>[3x]MEITTLQIVLVFIVACIAGMGSILDEFQFHRPLIACTLVGIVLGDMKTGIIIGGTLEMIALGWMNIGAAVAPDAALASIISTILVIAGHQSIGAGIALAIPLAAAGQVLTIIVRTITVAFQHAADKAADNGNLTAISWIHVSSLFLQAMRVAIPAVIVALSVGTSEVQNMLNAIPEVVTNGLNIAGGMIVVVGYAMVINMMRAGYLMPFFYLGFVTAAFTNFNLVALGVIGTVMAVLYIQLSPKYNRVAGAPAQAAGNNDLDNELDHHHHHHHH;>MVDTTQTTTEKKLTQSDIRGVFLRSNLFQGSWNFERMQALGFCFSMVPAIRRLYPENNEARKQ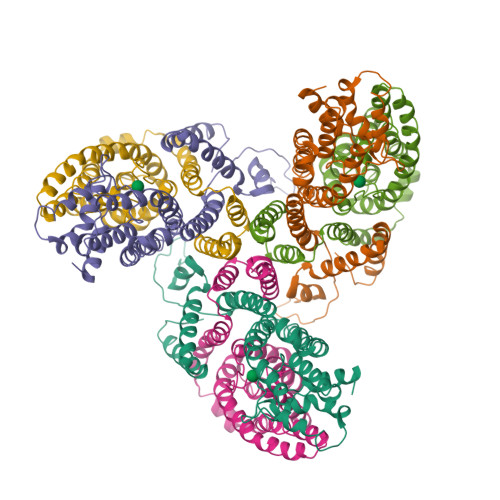AIRRHLEFFNTQPFVAAPILGVTLALEEQRANGAEIDDGAINGIKVGLMGPLAGVGDPIFWGTVRPVFAALGAGIAMSGSLLGPLLFFILFNLVRLATRYYGVAYGYSKGIDIVKDMGGGFLQKLTEGASILGLFVMGALVNKWTHVNIPLVVSRITDQTGKEHVTTVQTILDQLMPGLVPLLLTFACMWLLRKKVNPLWIIVGFFVIGIAGYACGLLGL[3x]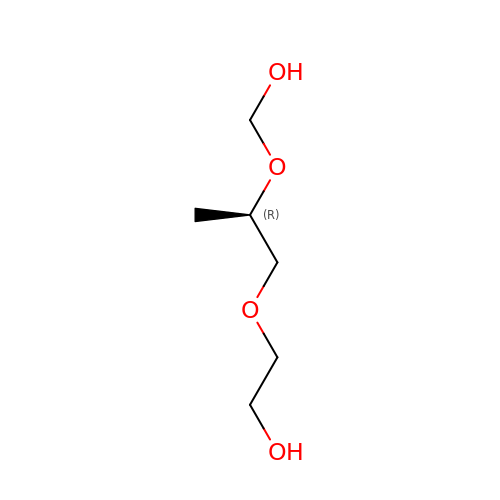2-[(2~{R})-2-(hydroxymethyloxy)propoxy]ethanol | C6 H14 O4 | DTSSVYVAVAHLGJ-ZCFIWIBFSA-N> GCGT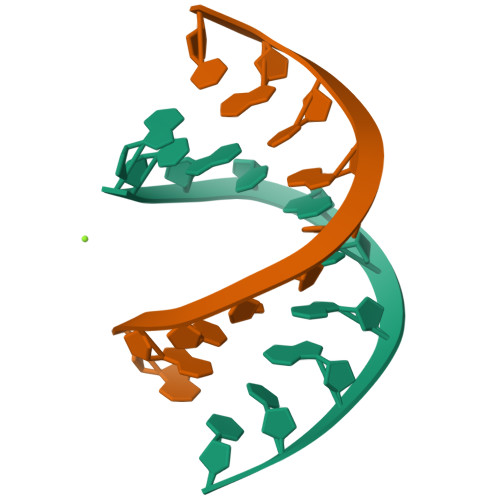GGGACC;> GGTCCCACGC>[2x]MLEDPGGRPRVYVDVREERSPVPSILESLGVQVIPKQ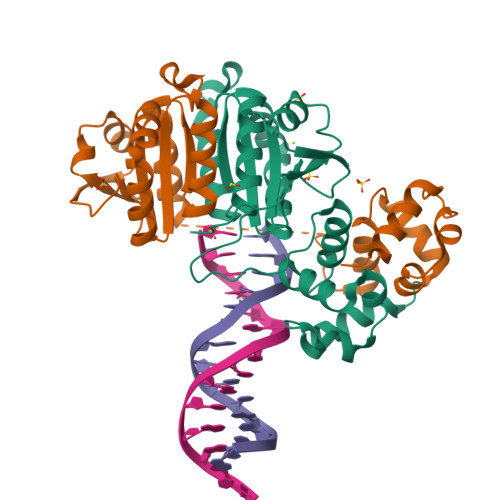LPMGDYLVSDSIIVERKTSSDFAKSLFDGRLFEQASRLAEHYETVFIIVEGPPVPRRYRGRERSLYAAMAALQLDYGIRLMNTMDPKGTALVIESLARLSTREGGQRIVIHKKPRLSDVREWQLYILQSFPGIGRRTAERILERFGSLERFFTASKAEISKVEGIGEKRAEEIKKILMTPYK> MNNQDALFPIVKDDIAFETLLTQAKTVIEQQSGQLWSNTEENDPGITLLEACCYGASDLAYRHSLPLRDLLTPEKQEQTLGDGIFPQEFGPQQMLTCGPITAEDYRRALLDLHSSDTDNETSEDYFFFNDVRLICEPESERYKYWYNKESREYSFIQEQEQEQEQLQLTLRGNYWLYLLPNRETEDDKTLTQKRLNDFLKDNRNLGESVSKIIWLQPVDFLLQLDIELDDDVSDLADIFAQVYMTTEQMVLTSPLRYSTQAMIEQGYSNEEIFEGPYLHHGWIPELSAAKDYTKPTELKLSHLANRLLAIPGVQNITRLALGKHDENISPLADDSWSWTIAQGYYPRLWGNDPLDLISSSASPLTITAKGGVKITVSKQDIENKIIAEPLIETQPELLNWGKHRKVLDYYPVSNKLPACYGLQTYAETQQQVHLHQFMLPFEQMLANGCAELALLPKLLAFKQRGNTVYGTQWPFKANTVGQQVHQEIMPDLIKQLNNDSQINSDDGIHSQNYTKELSILNYLLEYFGTHRAARPLTLDSLDFLSTQRGYLA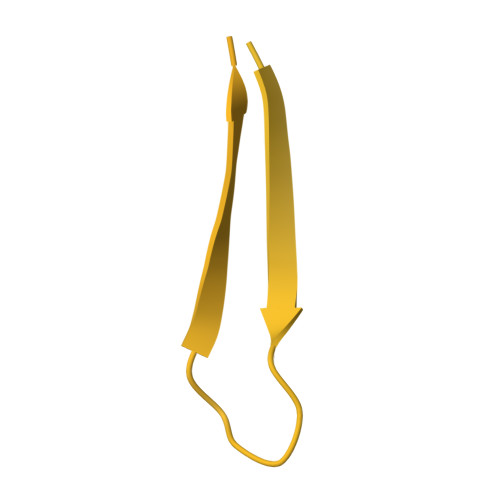QQPELTYQRNNIRIDKVSALQKRIAARLGLGGKCFEETSKLDELPFYLIEHRQLLPVKPDTKFDKEQKPDKLKIKSVPNSKNQQLIITQNGTTGQLLYGQVINLIIKEKENQDIRVKFILRGQMITDITGESFILDTRNSTALARSLIDVQNAYNDGNLYWCNSPVWMEDMDYQLVYASEIYQTGTENERWITSSPQSPFPAMIEENDEITLKYVITPSGPKKSDHELKANVIKFDRIQGKILIKLTQDSQDNFPLAADAWRYRWYFSSEKYALADRFSFVVSMVINSQLVKNDDVDPYKLESWAKTEILAEFPAHLSMIIHWLSPEDFKDFVSTYQRWQNNGAPLGDEAYHVLETLTLGRLPSAATGIGNMRIATAQQRIGVVGESGKEWNTEVIISNQLVYVPYTGENLNKR> MVERKPVFVDWCPGCGDFGILRAEEMAIRELGINPKSVVIVSGIGCSGKIPHFMNLPISGVHTLHGRSIAFATGIKLSNPSLEVIVNVGDGDGLGIGMGHFVHLGRRNIDIAVLVHNNGVYGLTKGQASPTLHRGEKTKSLPKPNIMDAVNPLAVALAAGYTFVARGYAYDVMHLKELIKKAILHKGSALVDILQPCPTYNDINTKEWYDKRVYK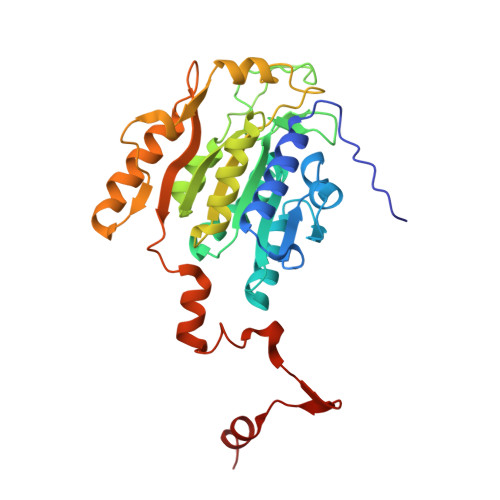LDNVPGWDPVVRKEEEAQKKFEQAIMKSYEWGEKIPIGIFYQNELVPTFEDRLTSNIPNYREYYPAKQQIEINGISTTKIDELIKAKRI> MSQRIIQPSASDQQFPGKSDGYEYTVGPKQAITSEASTTYIPSRIYSESLLFKRQEASLSAMAFLFQEMISQLHRTCKTAGDFETKLSDYGHNIGIRLLELLNFRASVSPSSLPRASAFLSQNESSSKLSNASNSPGMLANSSTATSASANERLQEKQTESLSNYITKMRRRDLKILDILQFIHGTLWSYLFNHVSDDLVKSSERDNEYMIVDNFPTLTQFIPGE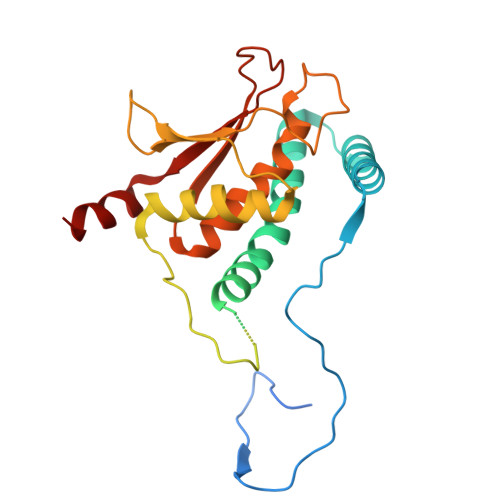NVSCEYFVCGIIKGFLFNAGFPCGVTAHRMPQGGHSQRTVYLIQFDRQVLDREGLRFG> HHHHHHGEVVNAACAVDAGSVDQTVQLGQVRTASLAQEGATSSAVGFNIQLNDCDTNVASKAAVAFLGTAIDAGHTNVLALQSSAAGSATNVGVQILDRTGAALTLDGATFSSETTLNNGTNTI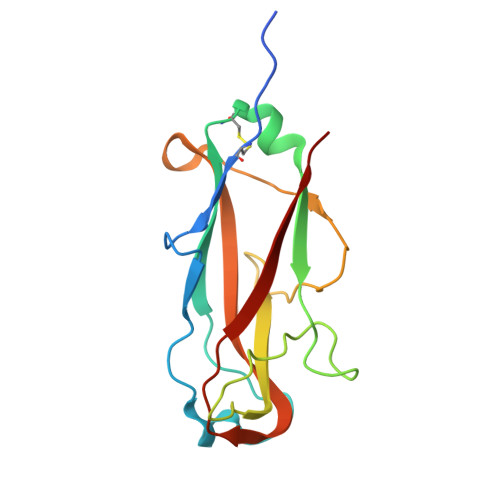PFQARYFATGAATPGAANADATFKVQYQ> MTHIAMSGLTNMQKYWLITGSVGPRPIALVTSLNSEGLCNAAPYSAFNYMGEDPPLFVIAVDHYGEESHRPGEQKDTLKNIIEREQFVVNMVDERIAE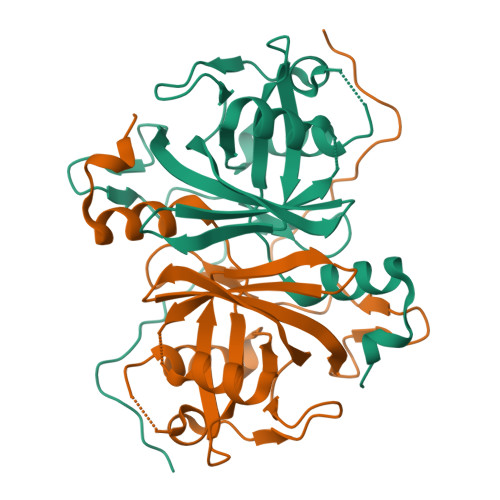RMVLCGSDFPSHISEAEAVGFDLTPSTTIDVPRITDAPIAWECKLYKIIDFSKQRSMVFGEIVAMYFREELIDEEKLRVRVDLFQPYGRLGGPNYCRTTDRVRLTVPTFLPSAGKPRE>MYGKLNKLVEHIKELLQQLNKNWHRHQGNLHDMNQQMEQLFQEFQHFMQGNQDDGKLQNMIHEMQQFMNQVDNHLQSESDTVHHFHNKLQELMNNFHHLV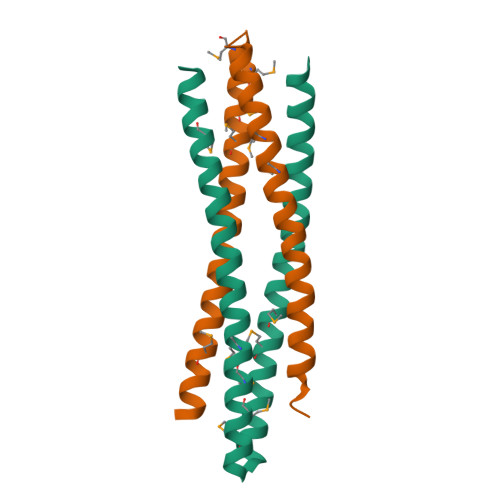HR[2x]>[2x]MGSSHHHHHHSSGLVPRGSMRGSHMPEGTLQLWTLQLAPKFNPYMDDVLGSWDKLHPEALVRWTDLPWGSVERKLLAAVFARTAPDVVNLNPPFAANLASKGGLTDLTALLPPGAEQNYLPSVWEAARDPEAGQIAIPWYLTVRLSLVNGDLLRQAGLSRAPRRWDEVPAYARSIRERTGRYGLFVTVVPDDSAELLESFVQMGVSLLDARQRAAF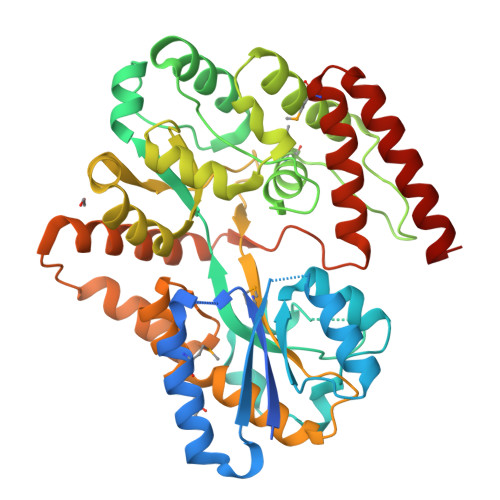NTPAGRKAFAFWTDLYREGLLPREVVSQGQRRAIELYQSGELALLASGAEFLRSIQTNAPGVAAVTTPQPPLTGSDGTANVALMTLAVPRQSQQAGEAVELALFLTNGTNQARFAREARVLPSSLEALSAIRAELEVEQPSNPAEAQIRDARLLSAETLNTARVLVPATPGVKRLQSIIYTQLQRAMLGQISSDQAVLEAEQQWNRYASARWP> STYPPTPPNVTRLSDESVMLRWMVPRNDGLPIVIFKVQYRMVGKRKNWQTTNDNIPYGKPKWNSELGKSFTASVTDLKPQHTYRFRILAVYSNNDNKESN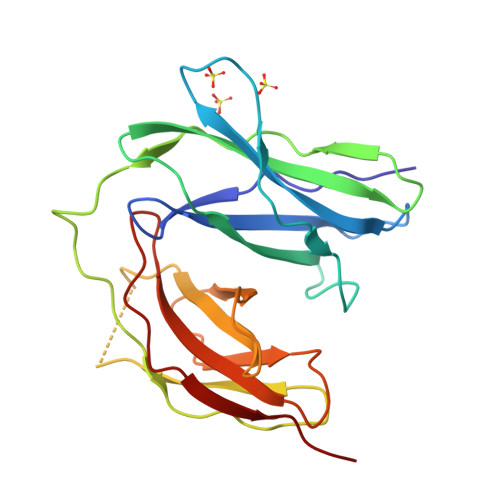TSAKFYLQPGAALDPMPVPELLEIEEYSETAVVLHWSLASDADEHLITGYYAYYRPSSSAGEYFKATIEGAHARSFKIAPLETATMYEFKLQSFSAASASEFSALKQGRTQRP> MSNQIYSARYSGVDVYEFIHSTGSIMKR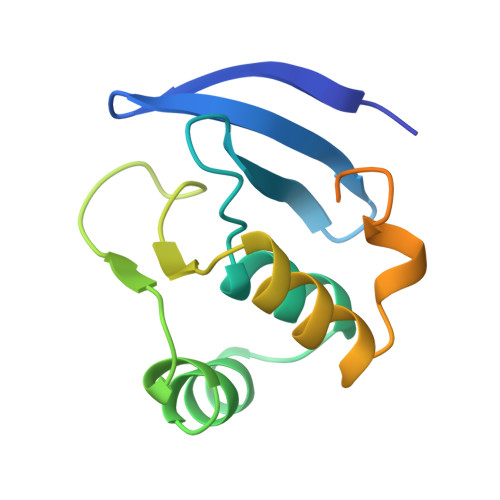KKDDWVNATHILKAANFAKAKRTRILEKEVLKETHEKVQGGFGKYQGTWVPLNIAKQLAEKFSVYDQLKPLFDFTQTDGSASPPPAPKHHHASKVDHHHHHH>MGQNHHEVVKFMDVYQRSYCHPIETLVDIFQEYPDEIEYIFKPSCVPLMRCGGCCNDEGLECVPTEESNITMQIMRIKPHQGQHIGEMSFLQHNKCECRPKKD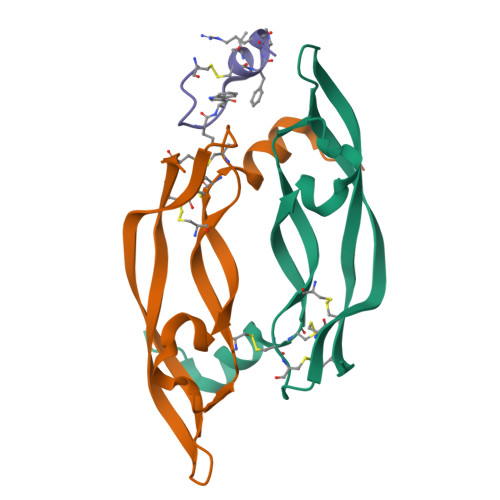[2x]> MSDSKCDSQFYSVQVADSTFTVLKRYQQLKPIGSGAQGIVCAAFDTVLGINVAVKKLSRPFQNQTHAKRAYRELVLLKCVNHKNIISLLNVFTPQKTLEEFQDVYLVMELMDANLCQVIHMELDHERMSYLLYQMLCGIKHLHSAGIIHRDLKPSNIVVKSDCTLKILDFGLARTACTNFMMTPYVVTRYYRAPEVILGMGYKENVDIWSVGCIMGELVKGCVIFQGTDHIDQWNKVIEQLGTPSAEFMKKLQPTVRNYVENRPKYPGIKFEELFPDWIFPSESERDKIKTSQARDLLSKMLVIDPDKRISVDEALRHPYITVWYDPAEAEAPPPQIYDAQLEEREHAIEEWKELIYKEVMDWEERSKNGVVKDQPSDAAVSSNATPSQSSSINDISSMSTEQTLASDTDSSLD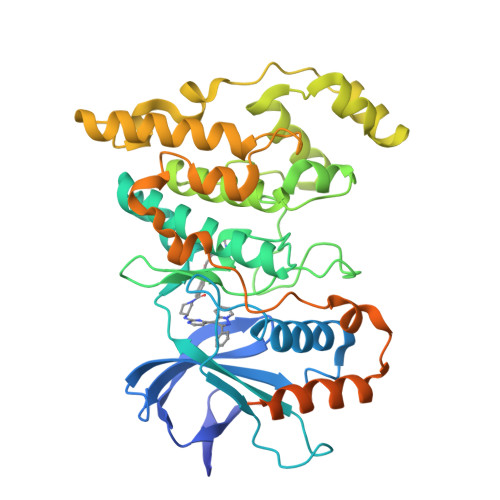ASTGPLEGCR>MWSHPQFEKASMVLMIVSGRSGSGKSVALRALEDMGFYCVDNLPVVLLPDLARTLADREISAAVSIDVRNMPESPEIFEQAMSNLPDAFSPQLLFLDADRNTLIRRYSDTRRLHPLSSKNLSLESAIDKESDLLEPLRSRADLIVDTSEMSVHELAEMLRTRLLGKRERELTMVFESFGFKHGIPIDADYVFDVRFLPNPHWDPKLRPMTGLDKPVAAFLDRHTEVHNFIYQTRSYLELWLPMLETNNRSYLTVAIGCTGGKHRSVYIAEQLADYFRSRGKNVQSRHRTLEKRKP[4x]

In phylogenetically diverse bacteria, the conserved protein RapZ plays a central role in RNA-mediated regulation of amino-sugar metabolism. RapZ contributes to the control of glucosamine phosphate biogenesis by selectively presenting the regulatory small RNA GlmZ to the essential ribonuclease RNase E for inactivation. Here, we report the crystal structures of full length Escherichia coli RapZ at 3.40 Å and 3.25 Å, and its isolated C-terminal domain at 1.17 Å resolution. The structural data confirm that the N-terminal domain of RapZ possesses a kinase fold, whereas the C-terminal domain bears closest homology to a subdomain of 6-phosphofructokinase, an important enzyme in the glycolytic pathway.

The refined model of RapZ-CTD was used to solve the crystal structure of the full-length protein by molecular replacement with the two previously collected X-ray diffraction datasets (space groups P32 and P3221). Four subunits of RapZ-CTD could be accommodated within the asymmetric unit of both datasets, and the calculated electron density map provided sufficient definition to manually build secondary structure features for the NTD starting from the CTD-based core of the tetrameric assembly. Overall, unambiguous electron density throughout most of each subunit chain allowed residues 1–281 to be modelled and refined. Areas for which electron density could not be observed include regions connecting the CTD and N-terminal domain (hereafter, NTD) of Chains C and D (residues 153–159) and a loop (residues 99–112) that is disordered in both Chains A and B. The same loop is, however, modelled in Chains C and D where the density was unambiguous. The overall topology and structural arrangement of RapZ is almost identical within the two distinct crystal forms. The tetrameric assembly is composed of a dimer of dimers in which the NTD and CTD form two homodimeric pairs. The CTD forms tightly packed dimers in a manner that exactly resembles the dimers seen in the RapZ-CTD structure. Interestingly the overall assembly is asymmetric as a consequence of flexibility in the NTD dimers. Moreover, the quaternary structure comprises a domain swapped dimer-of-dimers formed through the interlacing of the subunits. The crystal structures suggest that three distinct inter-protomer interfaces support the RapZ tetrameric assembly: the homotypic, symmetrical self-interactions between the N-terminal domain and the C-terminal domain, and two heterotypic interaction surfaces between the N- and C- terminal domains.> MSSMILTQFGPFIESISGITDQSNDVFEDAAKAFSMFTRSDVYKALDEIPFSDDAMLPIPPTIYTKPSHDSYYYIDALNRVRRKTYQGPDDVYVPNCSIVELLEPHETLTSYGRLSEAIENRAKDGDSQARIATTYGRIAESQARQIKAPLEKFVLALLVAEAGGSLYDPVLQKYDEIPDLSHNCPLWCFREICRHISGPLPDRAPYLYLSAGVFWLMSPRMTSAIPPLLSDLVNLAILQQTAGLDPSLVKLGVQICLHAAAS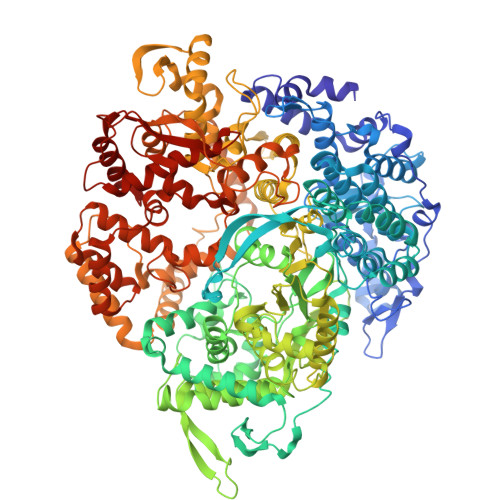SSYAWFILKTKSIFPQNTLHSMYESLEGGYCPNLEWLEPRSDYKFMYMGVMPLSAKYARSAPSNDKKARELGEKYGLSSVVGELRKRTKTYVKHDFASVRYIRDAMACTSGIFLVRTPTETVLQEYTQSPEIKVPIPQKDWTGPIGEIRILKDTTSSIARYLYRTWYLAAARMAAQPRTWDPLFQAIMRSQYVTARGGSGAALRESLYAINVSLPDFKGLPVKAATKIFQAAQLANLPFSHTSVAILADTSMGLRNQVQRRPRSIMPLNVPQQQVSAPHTLTADYINYHMNLSTTSGSAVIEKVIPLGVYASSPPNQSINIDISACDASITWDFFLSVIMAAIHEGVASSSIGKPFMGVPASIVNDESVVGVRAARPISGMQNMIQHLSKLYKRGFSYRVNDSFSPGNDFTHMTTTFPSGSTATSTEHTANNSTMMETFLTVWGPEHTDDPDVLRLMKSLTIQRNYVCQGDDGLMIIDGTTAGKVNSETIQKMLELISKYGEEFGWKYDIAYDGTAEYLKLYFIFGCRIPNLSRHPIVGKERANSSAEEPWPAILDQIMGVFFNGVHDGLQWQRWIRYSWALCCAFSRQRTMIGESVGYLQYPMWSFVYWGLPLVKAFGSDPWIFSWYMPTGDLGMYSWISLIRPLMTRWMVANGYVTDRCSPVFGNADYRRCFNELKLYQGYYMAQLPRNPKKSGRAAPREVREQFTQALSDYLMQNPELKSRVLRGRSEWEKYGAGIIHNPPSLFDVPHKWYQGAQEAAIATREELAEMDETLMRARRHSYSSFSKLLEAYLLVKWRMCEAREPSVDLRLPLCAGIDPLNSDPFLKMVSVGPMLQSTRKYFAQTLFMAKTVSGLDVNAIDSALLRLRTLGADKKALTAQLLMVGLQESEADALAGKIMLQDVNTVQLARVVNLAVPDTWMSLDFDSMFKHHVKLLPKDGRHLNTDIPPRMGWLRAILRFLGAGMVMTATGVAVDIYLEDIHGGGRSLGQRFMTWMRQEGRSA>[2x]SGFEFHGYARSGVIMNDSGASTKSGAYITPAGETGGAIGRLGNQADTYVEMNLEHKQTLDNGATTRFKVMVADGQ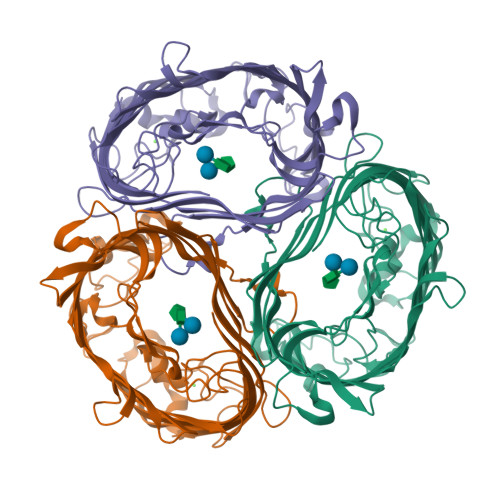TSYNDWTASTSDLNVRQAFVELGNLPTFAGPFKGSTLWAGKRFDRDNFDIHWIDSDVVFLAGTGGGIYDVKWNDGLRSNFSLYGRNFGDIDDSSNSVQNYILTMNHFAGPLQMMVSGLRAKDNDERKDSNGNLAKGDAANTGVHALLGLHNDSFYGLRDGSSKTALLYGHGLGAEVKGIGSDGALRPGADTWRIASYGTTPLSENWSVAPAMLAQRSKDRYADGDSYQWATFNLRLIQAINQNFALAYEGSYQYMDLKPEGYNDRQAVNGSFYKLTFAPTFKVGSIGDFFSRPEIRFYTSWMDWSKKLNNYASDDALGSDGFNSGGEWSFGVQMETWF;> SGFEFHGYAPSGVIMNDSGASTKSGAYITPAGETGGAIGPLGNAADTYVIMNLEHKQTLDNGATTRFKVMVADGQTSYNDWTASTSDLNVLQAFVELGNLPTFAGPFKGSTLWAGKRFDRDNFAIHWILSCVVFLAGTGGGIYDVKWNDGLRSNFSLYGRNFGDIDDSSNSVQNYILTMNHFAGPLQMMVSGLRAKDNDERKDSNGNLAKGDAANTGVHALLGLHNDSFYGLRDGSSKTALLYGHGLGAEVKGIGSDGALRPGADTWRIASYGTTPLSENWSVAPAMLAQRSKDRYADGDSYQWATFNLRLIQAINQNFALAYEGSYQYMDLKPEGYNDRQAVNGSFYKLTFAPTFKVGSIGDFFSRPEIRFYTSWMDWSKKLNNYASDDALGSDGFNSGGEWSFGVQMETAF> GWY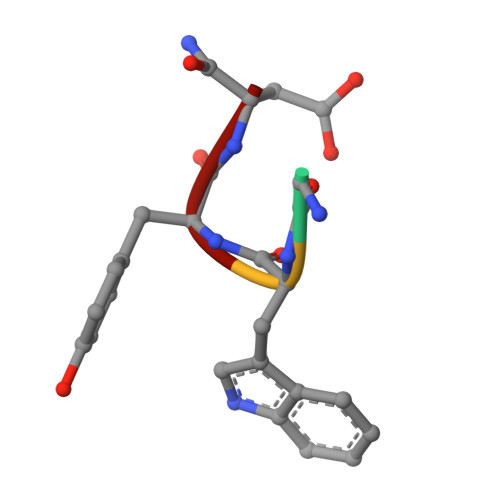N>[3x]GSVRPVVGEIAANSIAAEAQIAPGTE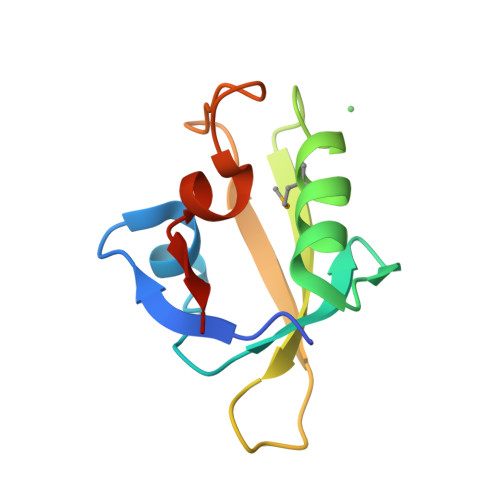LKAVDGIETPDWDAVRLQMVDKIGDESTTITVAPFGSDQRRDVKLDLRHWAFEPDKEDPVSSLGIRPRGPQ> SNTQAERSIIGMIDMFHKYTRRDDKIDKPSLLTMMKENFPNFLSACDKKGTNYLADVFEKKDKNEDKKIDFSEFLSLLGDIATDYHK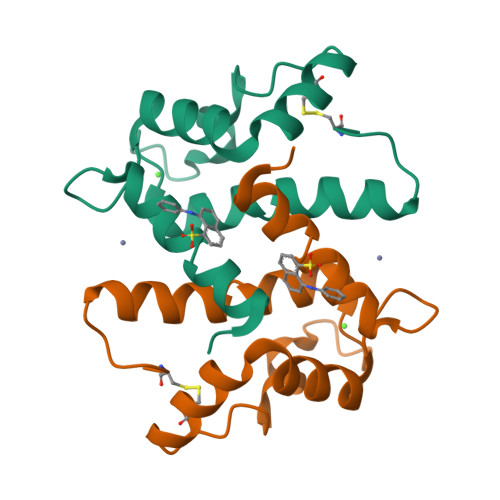QSHGAAPCSGGSQ>[2x]SAKELRCQCIKTYSKPFH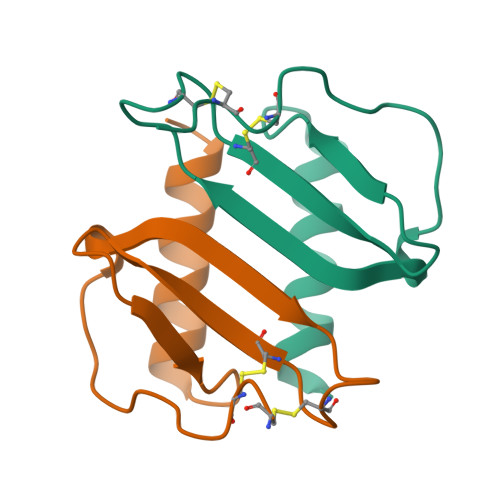PKFIKELRVIESGPHCANTCIIVKLSDGRELALDPKENWVQRVVEKFLKRAENS> KELAEKAGALAGEAARI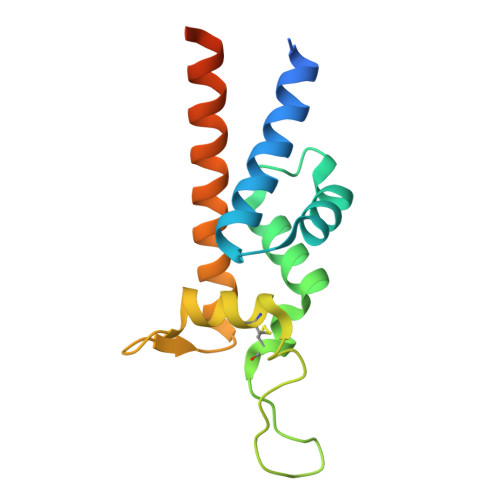PAAIDAVIEGIKSKFSIDTLGGEALKSVIDGTNYYDASYITTAIYNKFQVSSCLPSVPFLGGPPVPGAGANKPICSAVDKLYLGSGNFLDKSSLPGSIQKDVAKIVAGAEQAAKAKAAMVASDKTLAVETAKKQ>LTEQQRRELDWEKTDGLMPVIVQHAVSGEVLMLGYMNPEALDKTIESGKVTFFSRTKQRLWIKGETSGNFLNVVSIAPDCDNDTLLVLANPIGPTCHKGTSSCFGNTAHQWLFLYQLEQLLAERKYADPETSYTAKLYASGTKRIAQKMGEEGV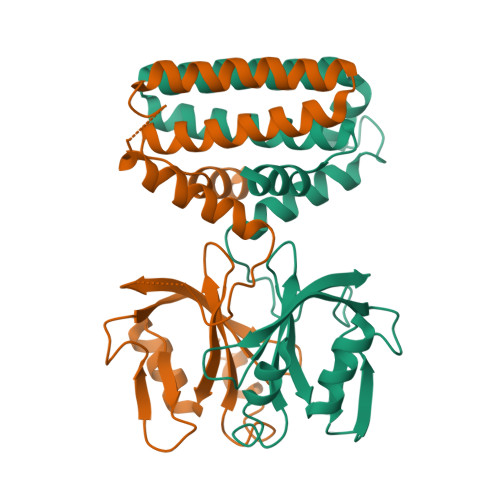ETALAATVHDRFELTNEASDLMYHLLVLLQDQDLDLTTVIENLHKRHQ[2x]> VDDDDKIVGGYTCGANTVPYQVSLNSGYHFCGGSLINSQWVVSAAHCYKSGIQVRLGEDNINVVEGNEQFISASKSIVHPSYNSNTLNNDIMLIKLKSAASLNSRVASISLPTSCASAGTQCLISGWGNTKSSGTSYPDVLKCLKAPILSDSSCKSAYPGQITSNMFCAGYLEGGKDSCQGDSGGP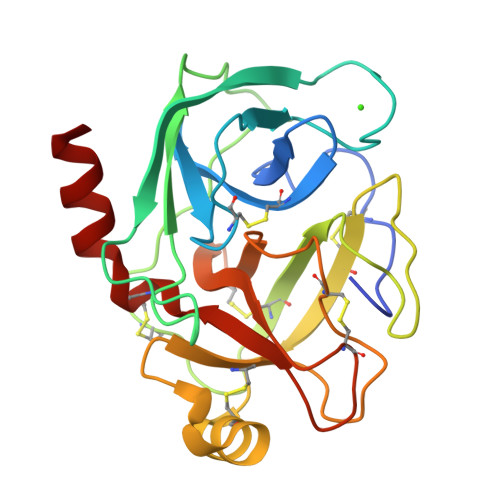VVCSGKLQGIVSWGSGCAQKNKPGVYTKVCNYVSWIKQTIASN> MQEGQNRKTSSLSILAIAGVEPYQEKPGEEYMNEAQLAHFRRILEAWRNQLRDEVDRTVTHMQDEAANFPDPVDRAAQEEEFSLELRNRDRERKLIKKIEKTLKKVEDEDFGYCESCGVEIGIRRLEARPTADLCI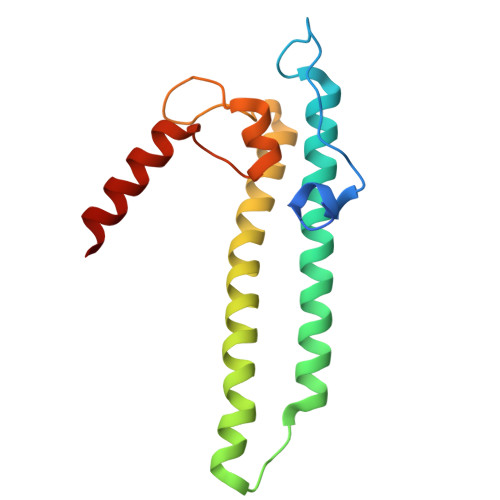DCKTLAEIREKQMAG> MEAILSKMKEVVENPNAAVKKYKSETGKKAIGCFPVYCPEEIIHAAGMLPVGIWGGQTELDLAKQYFPAFACSIMQSCLEYGLKGAYDELSGVIIPGMCDTLICLGQNWKSAVPHIKYISLVHPQNRKLEAGVKYLISEYKGVKRELEEICGYEIEEAKIHESIEVYNEHRKTMRDFVEVAYKHSNTIKPS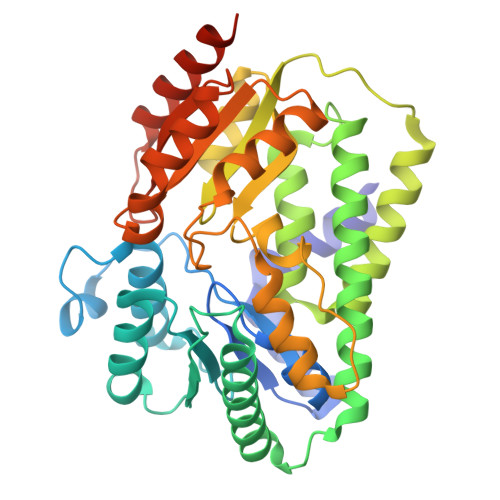IRSLVIKSGFFMRKEEHTELVKDLIAKLNAMPEEVCSGKKVLLTGILADSKDILDILEDNNISVVADDLAQETRQFRTDVPAGDDALERLARQWSNIEGCSLAYDPKKKRGSLIVDEVKKKDIDGVIFCMMKFCDPEEYDYPLVRKDIEDSGIPTLYVEIDQQTQNNEQARTRIQTFAEMMSLASAWSHPQFEK4-heptylbenzoic acid | C14 H20 O2 | 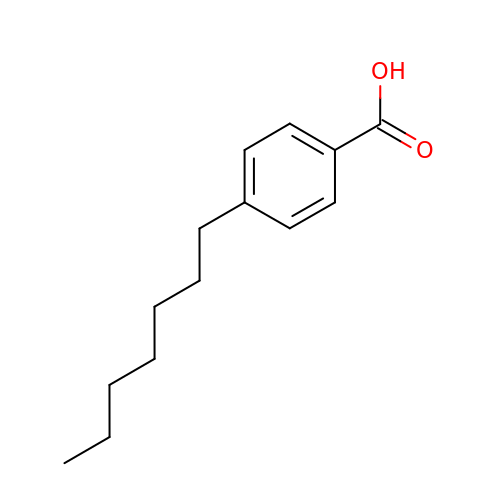VSUKEWPHURLYTK-UHFFFAOYSA-N> MKTVTVKNLIIGEGMPKIIVSLMGRDINSVKAEALAYREATFDILEWRVDHFMDIASTQSVLTAARVIRDAMPDIPLLFTFRSAKEGGEQTITTQHYLTLNRAAIDSGLVDMIDLELFTGDADVKATVDYAHAHNVYVVMSNHDFHQTPSAEEMVSRLRKMQALGADIPKIAVMPQSKHDVLTLLTATLEMQQHYADRPVITMSMAKEGVISRLAGEVFGSAATFGAVKQASAPGQIAVND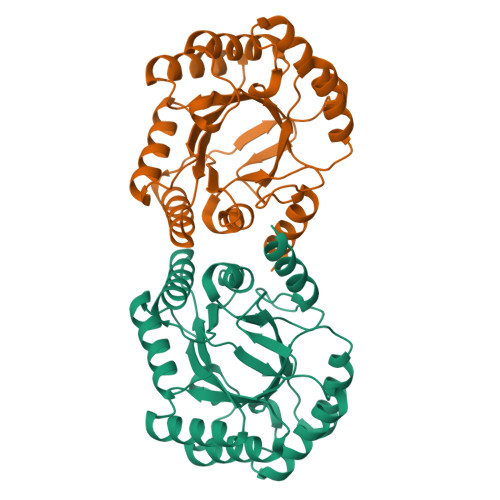LRSVLMILHNA>[2x]MVKMIVGLGNPGSKYEKTKHN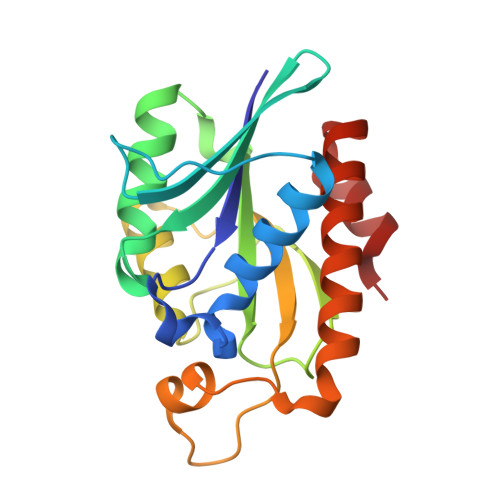IGFMAIDNIVKNLDVTFTDDKNFKAQIGSTFINHEKVYFVKPTTFMNNSGIAVKALLTYYNIDITDLIVIYDDLDMEVSKLRLRSKGSAGGHNGIKSIIAHIGTQEFNRIKVGIGRPLKGMTVINHVMGQFNTEDNIAISLTLDRVVNAVKFYLQENDFEKTMQKFNG5-{2-[1-(5-HYDROXY-1,5-DIMETHYL-HEXYL)-7A-METHYL-OCTAHYDRO-INDEN-4-YLIDENE]-ETHYLIDENE}-2-METHYL-CYCLOHEXANE-1,3-DIOL 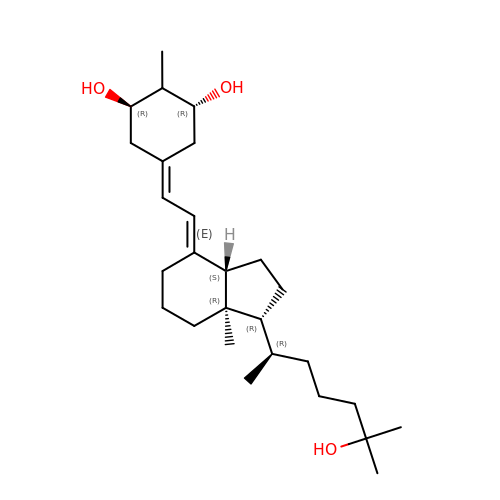| C27 H46 O3 | OZPNRDQPQFOURL-VJPYOZRWSA-N> GVALGATRVIYPAGQKQEQLAVTNNDENSTYLIQSWVENADGVKDGRFIVTPPLFAMKGKKENTLRILDATNNQLPQDRESLFWMNVKAIPSMDKSKLTENTLQLAIISRIKLYYRPAKLALPPDQAAEKLRFRRSANSLTLINPTPYYLTVTELNAGTRVLENALVPPMGESTVKLPSDAGSNITYRTINDYGALTPKMTGVMEHHHHHH;> DLYFNPRFLADDPQAVADLSRFENGQELPPGTYRVDIYLNNGYMATRDVTFNTGDSEQGIVPCLTRAQLASMGLNTASVAGMNLLADDACVPLTTMVQDATAHLDVGQQRLNLTIPQAFMSNRARGYIPPELWDPGINAGLLNYNFSGNSVQNRIGGNSHYAYLNLQSGLNIGAWRLRDNTTWSYNSSDRSSGSKNKWQHINTWLERDIIPLRSRLTLGDGYTQGDIFDGINFRGAQLASDDNMLPDSQRGFAPVIHGIARGTAQVTIKQNGYDIYNSTVPPGPFTINDIYAAGNSGDLQVTIKEADGSTQIFTVPYSSVPLLQREGHTRYSITAGEYRSGNAQQEKPRFFQSTLLHGLPAGWTIYGGTQLADRYRAFNFGIGKNMGALGALSVDMTQANSTLPDDSQHDGQSVRFLYNKSLNESGTNIQLVGYRYSTSGYFNFADTTYSRMNGYNIETQDGVIQVKPKFTDYYNLAYNKRGKLQLTVTQQLGRTSTLYLSGSHQTYWGTSNVDEQFQAGLNTAFEDINWTLSYSLTKNAWQKGRDQMLALNVNIPFSHWLRSDSK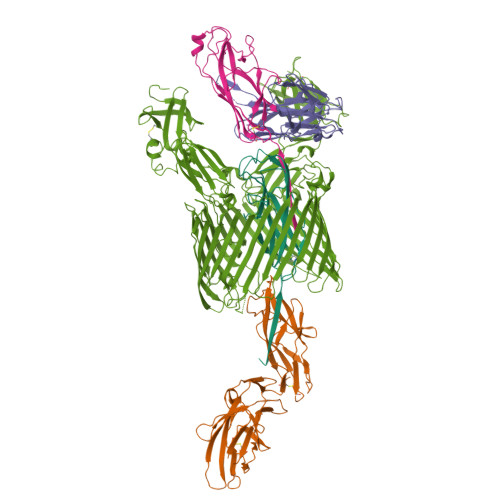SQWRHASASYSMSHDLNGRMTNLAGVYGTLLEDNNLSYSVQTGYAGGGDGNSGSTGYATLNYRGGYGNANIGYSHSDDIKQLYYGVSGGVLAHANGVTLGQPLNDTVVLVKAPGAKDAKVENQTGVRTDWRGYAVLPYATEYRENRVALDTNTLADNVDLDNAVANVVPTRGAIVRAEFKARVGIKLLMTLTHNNKPLPFGAMVTSESSQSSGIVADNGQVYLSGMPLAGKVQVKWGEEENAHCVANYQLPPESQQQLLTQLSAECRSAWSHPQFEK;> ADSTITIRGYVRDNGCSVAAESTNFTVDLMENAAKQFNNIGATTPVVPFRILLSPCGNAVSAVKVGFTGVADSHNANLLALENTVSAASGLGIQLLNEQQNQIPLNAPSSALSWTTLTPGKPNTLNFYARLMATQVPVTAGHINATATFTLEYQ;> ADVTITVNGKVVAKPCTVSTTNATVDLGDLYSFSLMSAGAASAWHDVALELTNCPVGTSRVTASFSGAADSTGYYKNQGTAQNIQLELQDDSGNTLNTGATKTVQVDDSSQSAHFPLQVRALTVNGGATQGTIQAVISITYTYS;> FACKTANGTAIPIGGGSANVYVNLAPVVNVGQNLVVDLSTQIFCHNDYPETITDYVTLQRGSAYGGVLSNFSGTVKYSGSSYPFPTTSETPRVVYNSRTDKPWPVALYLTPVSSAGGVAIKAGSLIAVLILRQTNNYNSDDFQFVWNIYANNDVVVPTGGCDVSARDVTVTLPDYPGSVPIPLTVYCAKSQNLGYYLSGTTADAGNSIFTNTASFSPAQGVGVQLTRNGTIIPANNTVSLGAVGTSAVSLGLTANYARTGGQVTAGNVQSIIGVTFVYQ> DGPYLQILEQPKQRGFRFRYVCEGPSHGGLPGASSEKNKKSYPQVKICNYVGPAKVIVQLVTNGKNIHLHAHSLVGKHCEDGVCTVTAGPKDMVVGFANLGILHVTKKKVFETLEARMTEACIRGYNPGLLVHSDLAYLQAEGGGDRQLTDREKEIIRQAAVQQTKEMDLSVVRLMFTAFLPDSTGSFTRRLEPVVSDAIYDSKAPNASNLKIVRMDRTAGCVTGGEEIYLLCDKVQKDDIQIRFYEEEENGGVWEGFGDFSPTDVHRQF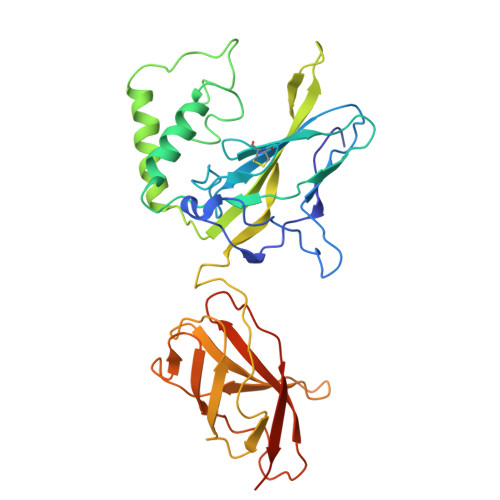AIVFKTPKYKDVNITKPASVFVQLRRKSDLETSEPKPFLYYPEIKDKEEVQRKRQK> MSHSLTSVFQKIDSLKPQFFSRLTKAIQIPAVSSDESLRSKVFDKAKFISEQLSQSGFHDIKMVDLGIQPPPISTPNLSLPPVILSRFGSDPSKKTVLVYGHYDVQPAQLEDGWDTEPFKLVIDEAKGIMKGRGVTDDTGPLLSWINVVDAFKASGQEFPVNLVTCFEGME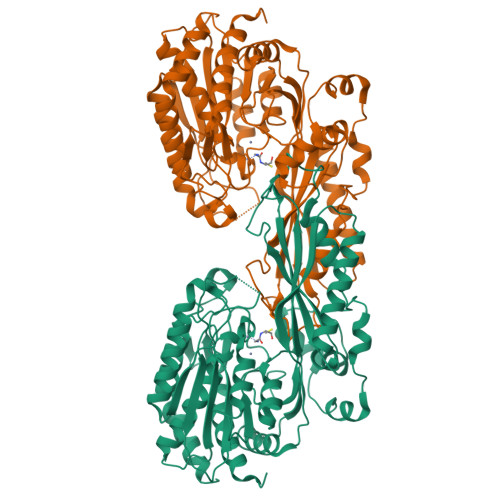ESGSLKLDELIKKEANGYFKGVDAVCISDNYWLGTKKPVLTYGLRGCNYYQTIIEGPSADLHSGIFGGVVAEPMIDLMQVLGSLVDSKGKILIDGIDEMVAPLTEKEKALYKDIEFSVEELNAATGSKTSLYDKKEDILMHRWRYPSLSIHGVEGAFSAQGAKTVIPAKVFGKFSIRTVPDMDSEKLTSLVQKHCDAKFKSLNSPNKCRTELIHDGAYWVSDPFNAQFTAAKKATKLVYGVDPDFTREGGSIPITLTFQDALNTSVLLLPMGRGDDGAHSINEKLDISNFVGGMKTMAAYLQYYSESPENHHHHHH>MEDINFASLAPRHGSRPFMGTWNEIGTSQLNGGAFSWSSLWSGIKNFGSSIKSFGNKAWNSNTGQMLRDKLKDQNFQQKVVDGLASGINGVVDIANQALQNQINQRLENSRQPPVALKQRPTPEPEEVEVEEKLPPLETAPPLPSKGEKRPRPELEETLVVESREPPSYEQALKEGASYPMTRPIGSMARPVYGKEKTPVTLELPPPAPTVPPMPTPTLGTNVPRLAAPTVAVATPARRVRGANWQSTLNSIVGLGVKSLKRRRCY[10x];>MATPSMMPQWSYMHIAGQDASEYLSPGLVQFARATDTYFSLGNKFRNPTVAPTH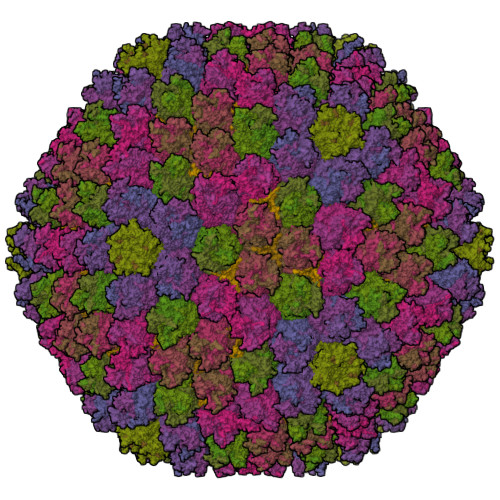DVTTDRSQRLTLRFVPVDREDTAYSYKVRFTLAVGDNRVLDMASTYFDIRGVLDRGPSFKPYSGTAYNSLAPKTAPNPCEWKDNNKIKVRGQAPFIGTNINKDNGIQIGTDTTNQPIYADKTYQPEPQVGQTQWNSEVGAAQKVAGRVLKDTTPMLPCYGSYAKPTNEKGGQASLITNGTDQTLTSDVNLQFFALPSTPNEPKAVLYAENVSIEAPDTHLVYKPDVAQGTISSADLLTQQAAPNRPNYIGFRDNFIGLMYYNSTGNMGVLAGQASQLNAVVDLQDRNTELSYQLMLDALGDRSRYFSMWNQAVDSYDPDVRIIENHGVEDELPNYCFPLGGSAATDTYSGIKANGQTWTADDNYADRGAEIESGNIFAMEINLAANLWRSFLYSNVALYLPDSYKITPDNITLPENKNTYAYMNGRVAVPSALDTYVNIGARWSPDPMDNVNPFNHHRNAGLRYRSMLLGNGRYVPFHIQVPQKFFAIKNLLLLPGSYTYEWNFRKDVNMILQSSLGNDLRVDGASVRFDSINLYANFFPMAHNTASTLEAMLRNDTNDQSFNDYLCAANMLYPIPSNATSVPISIPSRNWAAFRGWSFTRLKTKETPSLGSGFDPYFTYSGSVPYLDGTFYLNHTFKKVSIMFDSSVSWPGNDRLLTPNEFEIKRTVDGEGYNVAQCNMTKDWFLIQMLSHYNIGYQGFYVPESYKDRMYSFFRNFQPMSRQVVNTTTYKEYQNVTLPFQHNNSGFVGYMGPTMREGQAYPANYPYPLIGQTAVPSLTQKKFLCDRTMWRIPFSSNFMSMGALTDLGQNMLYANSAHALDMTFEVDPMDEPTLLYVLFEVFDVVRIHQPHRGVIEAVYLRTPFSAGNATT[12x];> MRRAVGVPPVMAYAEGPPPSYESVMGSADSPATLEALYVPPRYLGPTEGRNSIRYSELAPLYDTTRVYLVDNKSADIASLNYQNDHSNFQTTVVQNNDFTPAEAGTQTINFDERSRWGADLKTILRTNMPNINEFMSTNKFKARLMVEKKNKETGLPRYEWFEFTLPEGNYSETMTIDLMNNAIVDNYLEVGRQNGVLESDIGVKFDTRNFRLGWDPVTKLVMPGVYTNEAFHPDIVLLPGCGVDFTQSRLSNLLGIRKRLPFQEGFQIMYEDLEGGNIPALLDVAKYEASIQKAKEEGKEIGDDTFATRPQDLVIEPVAKDSKNRSYNLLPNDQNNTAYRSWFLAYNYGDPKKGVQSWTLLTTADVTCGSQQVYWSLPDMMQDPVTFRPSTQVSNYPVVGVELLPVHAKSFYNEQAVYSQLIRQSTALTHVFNRFPENQILVRPPAPTITTVSENVPALTDHGTLPLRSSISGVQRVTITDARRRTCPYVHKALGIVAPKVLSSRTF;> MSKRKFKEELLEALVPEIYGPAADVKPDIKPRALKRVKKREKKEETGLLDDDVEFVRTFAPRRQVQWRGRKVKRVLRPGTTVVFTPGERSATRALKREYDEVYADEDILEQAAQQIGEFAYGKRGRYGEVGLLLDQSNPTPSLKPATQQQILPVTETKRGVKRENKDELQPTMQLMVPKRQKLEEVLENMKVDPSVEPEVKVRPIKEIGPGLGVQTVDIQIPVRTTPAVAMAEAMETQTDQPAAVTTREIGLQTDPRYESVTSTRRSRGRKYTAANSILPEYALHPSITPTPGYRGTIFRPSRPRTTRRRRTTRRRSRRITPISVHRVTRRGRTITLPNARYHPSILI;> MQRSTAVVDGSQQVDPAMLAALQSQPSGVTPSDDWAAAMDRILALTTRNPEAFRQQPQANRFSAILEAVVPSRTNPTHEKVLAIVNALTESKAIRKDEAGLIYNALLERVARYNSTNVQANLDRLTTDVREAVAQRERFMHDTNLGSQVALNAFLSTLPANVPRGQEDYVSFISALRLLVAEVPQSEVYQSGPDYFFQTSRQGLQTVNLTQAFKNLQGMWGVRAPVGDRATISSLLTPNTRLLLLLIAPFTNSSTISRDSYLGHLITLYREAIGQTQVDEQTFQEITSVSRALGQQDTGSLEATLNFLLTNRQQKIPSQFTLSTEEERILRYVQQSVSLYLMREGMTPSSALDMTARNMEPSLYSSNRPFINRLMDYLHRAAAMNSEYFTNAILNPHWMPPSGFYTGEFDMPEGDDGFLWDDVSDSIFVPARYRKKEGGDELPLPLVEAASRGQSPFPSLPSLVSSSNSGRVLRPRLPGETDYLNDPLLQPVRNKNFPNNGVESLVDKMNRWKTYAQEQREWEESQSRPLAGPFSRWRRREDDQDDSADDNSVLDLGGTGASSNPFAHLRPQGRLGRLY;>[4x]MSGSMEGNAVSFKGGVFSPYLTTRLPAWAGVRQNVMGSNVDGRPVAPANSATLTYATVGSSVDTAAAAAASAAASTARGMAADFGLYNQLAASRSLREEDALSVVLTRLEELSQQLQDLFAKVALLNPPANAS;>MSKEIPTPYMWSYQPQMGLAAGASQDYSSRMNWLSAGPHMIGRVNGIRATRNQILLEQAALTSTPRSQLNPPNWPAAQVYQENPAPTTVLLPRDAEAEVQMTNSGAQLAGGSRHVRFRGRSSPYSPGPIKRLIIRGRGIQLNDEVVSSLTGLRPDGVFQLGGAGRSSFTPRQAYLTLQSSSSQPRSGGIGTLQFVEEFVPSVYFNPFSGAPGLYPDDFIPNYDAVSESVDGYD[2x];> FNPVYPY N-(6-oxo-6,9-dihydro-3H-purin-2-yl)acetamide | 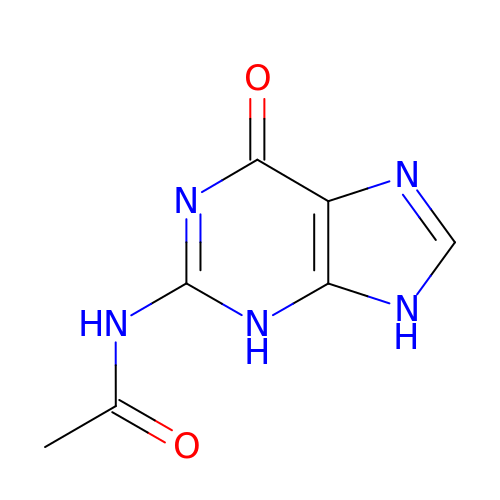C7 H7 N5 O2 | MXSMRDDXWJSGMC-UHFFFAOYSA-N> MKVETKRQRYNKRLHALKTERSSWEGSWRDISDHIQPWRSRFCMSDSNKGNRHNKALVDDTPFKASRTLASGMMSGLTSPARPWFKLAIDNPELMESAAVKQWLYLVTQRMQSVMSKSNLYNQLHQLYGELGTFGTSCILIVEDKEDVIRAIPMTVGTYYLATSSRGMVDTIYREMRKTVRQLVQEFGLKNCSNSVQTMYDNDNLEAWVEVVHLIEPNDERNEGKLDSKNKPYRSVYYESGCTEDKLLRESGFDEFPGVAPRWEVLGDDVYGYGPGHAALGPSRSLQVMQKKKAQAVEKQINPPMNVPSSSKSKPFSLLPGSLNYYDAAMGGQQMAQPSQSVNLNLNSIMEDIVAHQTSIKETFYADLFMMIANDQRSNITAREIQERHEEKLLALGPVVERLDTEALDPMIDRVFGIMMRGGHLPPPPEEIQGVDLNVQYISVMAQAQKLVGIG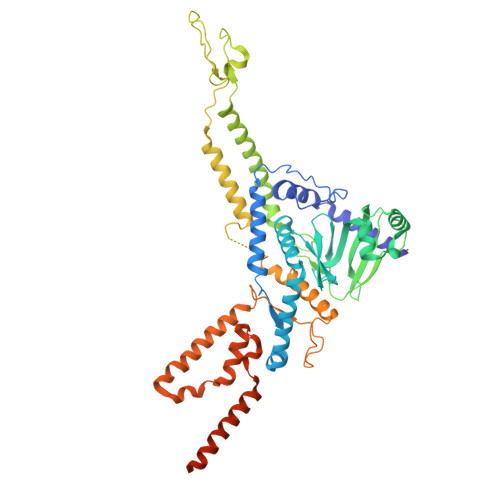AIERITSFVGNLAGADPSALDKLNIDQAIDQYSNSVSAPPDIIRTDDEVAEIRQARAQQQQQAQAMEMAQQAAQGAKLLSETDAGTGQNGLSAMMQQMGLA1,1-DIMETHYL-PROLINIUM | C7 H14 N 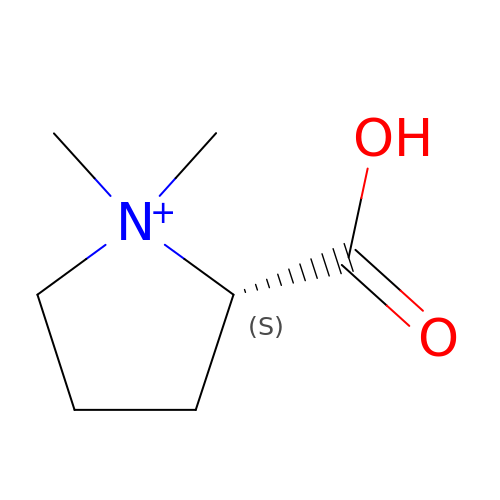O2 | CMUNUTVVOOHQPW-LURJTMIESA-O>[2x]MMSDQENENEHAKAFLGLAKCEEEVDAIEREVELYRLNKMKPVYEKRDAYIDEIAEFWKIVLSQHVSFANYIRASDFKYIDTIDKIKVEWLALESEMYDTR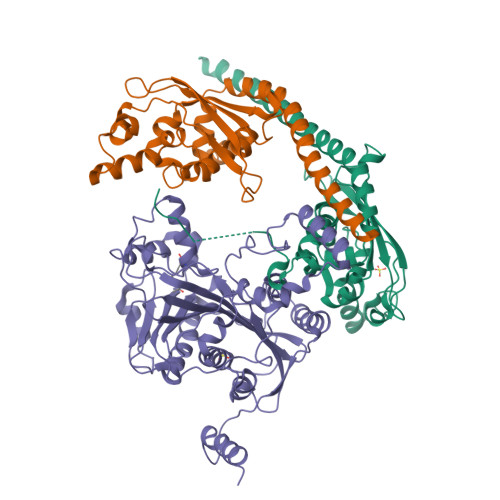DFSITFHFHGIEGDFKEQQVTKVFQIKKGKDDQEDGILTSEPVPIEWPQSYDSINPDLIKDKRSPEGKKKYRQGMKTIFGWFRWTGLKPGKEFPHGDSLASLFSEEIYPFCVKYYAEAQRDLEDEEGESGLSADGDSEDDDGSLGEVDLPLSDEEPSSKKRKV;> GMDPNSMSLNDFLSSVLPVSEQFEYLSLQSIPLETHAVVTPNKDDKRVPKSTIKTQHFFSLFHQGKVFFSLEVYVYVTLWDEADAERLIFVSKADTNGYCNTRVSVRDITKIILEFILSIDPNYYLQKVKPAIRSYKKISPELISAASTPARTLRILARRLKQSGSTVLKEIESPRFQQDLYLSFTCPREILTKICLFTRPASQYLFPDSSKNSKKHILNGEELMKWWGFILDRLLIECFQNDTQAKLRIPGEDPARVRSYLRGMKYPLWQVGDIFTSKENSLAVYNIPLFPDDPKARFIHQLAEEDRLLKVSLSSFWIELQERQEFKLSVTSSVMGISGYSLATPSLFPSSADVIVPKSRKQFRAIKKYITGEEYDTEEGAIEAFTNIRDFLLLRMATNLQSLTGKREHRERNQPVPASNINTLAITMLKPRKKAKALPKT>MSKEVVSLFFQASHDNDVETAMSCFAEDGIWVDPTGKVYERNEIKEYLVQQIGVLEDFHSQGVSVNYFDMVEAPDGRVYIGASVKAADGTEIRRFLDVFEMRDGKIAVKDVF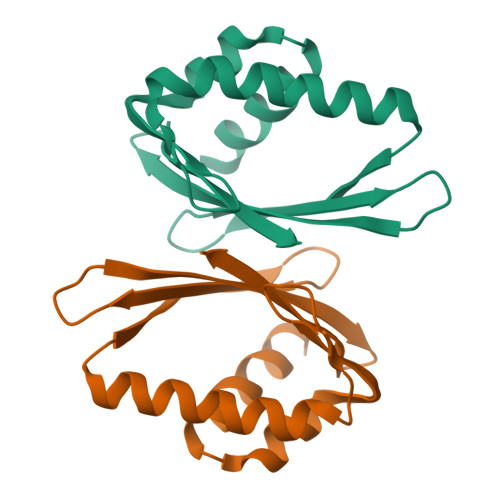GKQKLAAALEHHHHHH[4x]> MAHHHHHHMLPVHLKHPHLTATEEYLSEFWSEIAAQTIDWIQPWSITLQGGLHKGDVKWFQGGLLNVSANCLDRHLPHKANQTAIIWEGDDENQNKTLTFAQLYSEVCKMSNVLKSLNVRRGDTVGIYLPMIPEAAIAMLACARIGAIHTVVFAGFSAHALQQRLIASSCKCLITADAFQRGGKTIPLKKQADEASVDLNITKLVVKNSNAPTALNKNKEHWWHELKQTVSDQCTPEPMNTEDPLFILYTSGSTGQPKGVVHTTGGYLVQAAYTHQLIFACQDNEVFWCTADVG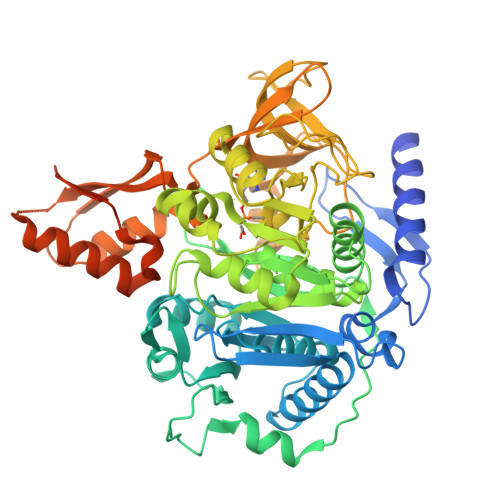WITGHSYVVYGPLCNGITTLMFEGIPTWPDAARNWRIIDKHQVNVFYTAPTAIRSLMRAGDQWLNSSSRSSLRLLGSVGEPINPEAWNWYHQKVGQGKCPIVDTWWQTETGAIMISPRASDEVIKPGSARKPIPGIVPLLLNEQGHEINGAGEGLLAIKYPWPSMARTIAGDHQRYCNTYLSNGYYITGDGAKRDEDGDYWITGRIDDVLNVSGHRLGTAEIESALVSHPKVAEAGVVGIPHDLKGQAIFAYVILKQGNKPDAELQTELMERVKDQISAIAKPDVIQFANDLPKTRSGKIMRRILRKIACKEVSHIDELGDLTTLANPQIVEELMKNILKR Hair cells have a characteristic morphology and harbor actin-filled stereocilia ‘staircases’ in which the stereocilia are coupled by protocadherin 15 (PCDH15) molecules from one stereocilium linked with cadherin 23 (CDH23) molecules from an adjacent stereocilium. Upon movement of the stereocilia induced by fluctuations of the surrounding fluid, the PCDH15-CDH23 ‘tip links’ trigger the opening of a mechano-electrical transduction (MET) ion channel at the stereocilia tips. PCDH15 belongs to the cadherin superfamily and consists of 11 extracellular cadherin (EC) domains, an extracellular linker (EL) domain, a single transmembrane (TM) helix and a cytoplasmic domain. Here we demonstrate that PCDH15 forms a robust complex with LHFPL5 and that the assembly is composed of 2 copies of each protein, thus providing concrete evidence that the composition of PCDH15 in the tip link is a dimer.

To screen for interaction partners of PCDH15 we created a PCDH15 construct where we deleted seven of the eleven cadherin repeats as well as the C-terminal region that differs between isoforms (PCDH154EC), arriving at a PCDH15 complex that retained important regions of the extracellular, transmembrane and cytoplasmic domains yet that also possessed monodisperse biochemical behavior. Imaging of the PCDH154EC-LHFPL5 complex by cryo-EM using a Volta phase plate showed particles composed of a micelle-shaped feature with two emerging strands, where the strands adopt a range of conformations. Analysis of these particles, deemed the ‘straight’ conformation, by 2D classification yields classes consistent with two cadherin chains adopting an approximately parallel configuration (green). We proceeded to carry out a 3D reconstruction and computed a reconstruction at ~11.3 Å resolution of this straight conformation (Figure 2—figure supplements 1 and 2c and d). The two density features protruding from the micelle are ~190 Å in length and ~20 Å in diameter, consistent with an approximately linear chain of four cadherin domains. At the base of the protruding density, proximal to the micelle, is a disk-shaped density that appears to be formed by the C-terminal part of EC11 and the ~100 residue EL domain. We were unable to fit this conformation of EC9-EC10 into our density map and therefore fitted EC8, EC9, and EC10 as independent rigid bodies, guided by the shape complementarity of the rigid-body docked domains. We observe a dimer interface between the two cadherin strands formed by the C-terminal half of EC9, largely defined by a loop between β1 and β2 strands and the N-terminus of the α-helix between β3 and β4. This interface appears to stabilize the straight conformation. The model shows that the 4 cadherin domains stretch 220 Å above the membrane, with the EC11-EL domain positioned ~27 Å above the TM region. The cadherin domains have a right handed twist of 23.9° from EC11 to EC8, consistent with a right-handed coil of the tip link observed in high-resolution EM imaging.

>[2x]QYDDSPVFTNSTYTVVVEENLPAGTSFLQIEAKDVDLGANVSYRIRSPEVKHLFALHPFTGELSLLRSLDYEAFPDQEASITFLAEAFDIYGTMPPGIATVTVIVKDMNDYPPVFSKRIYKGMVAPDAVKGTPITTVYAEDADPPGMPASRVRYRVDDVQFPYPASIFDVEEDSGRVVTRVNLNEEPTTIFKLVVVAFDDGEPVMSSSATVRILVLHPGEIPRFTQEEYRPPPVSELAARGTVVGVISAAAINQSIVYSIVAGNEEDKFGINNVTGVIYVNSPLDYETRTSYVLRVQADSLEVVLANLRVPSKSNTAKVYIEIQDENDHPPVFQKKFYIGGVSEDARMFASVLRVKATDRDTGNYSAMAYRLIIPPIKEGKEGFVVETYTGLIKTAMLFHNMRRSYFKFQVIATDDYGKGLSGKADVLVSVVNQLDMQVIVSNVPPTLVEKKIEDLTEILDRYVQEQIPGAKVVVESIGARRHGDAYSLEDYSKCDLTVYAIDPQTNRAIDRNELFKFLDGKLLDINKDFQPYYGEGGRILEIRTPEAVTSIKKRGESLGYTEGALLALAFIIILCCIPAILVVLVSYRQFKVRQAECTKTARIQSAMPAAKPAAPVPAAPAPPPPPPPPPPGAHLYEELGESAMHKYETALFESRLVPR>[2x]CGCAAATTXGCG

Using several techniques, we show that electron paramagnetic resonance (EPR) spectroscopy of oligonucleotides spin-labelled with triazole-appended nitroxides at the 2′ position offers a robust and minimally perturbing tool for obtaining such measurements. Here we address this challenge through a synergistic combination of EPR spectroscopy, X-ray crystallography, NMR spectroscopy and MD simulations, which accurately identify spin label location on a DNA duplex. As well as affording the first X-ray crystallographic structures of B-form spin-labelled DNA duplexes, the combination of these four techniques demonstrates the minimally perturbing nature of deoxynucleic acid 2′-spin-labelling. Using experimental and computational methods to support EPR spectroscopic observations, we demonstrate that spin-labelling of DNA via 2′-triazole-linked nitroxides is minimally perturbing and affords DEER data with narrow (sub-nanometre) distance distributions due to well-defined minor groove nitroxide conformations.

Copper-catalysed azide-alkyne cycloaddition with a tetramethylpyrrolinoxyl radical (‘5-Me’, 3) or a tetramethylpiperidinoxyl radical (‘6-Me’, 4) afforded duplexes 5 (containing two 5U modifications) and 6 (two 6U modifications). Notably, 6 adopts the B-form; prior to this work, the only reported crystal structure of spin-labelled DNA is in the A-form. The electron density of the 6-Me spin labels is well defined, with both modifications occupying the minor groove. The separation of the spin labels (measured from the centre of each N–O bond) is 2.87 nm, which is in good agreement with the most probable distance determined by EPR spectroscopy (2.99 nm). The electron density of all other residues is also well defined, except for the 5′-terminal 2′-deoxycytidines, whose base-pairing is disrupted by crystal-packing interactions with cobalt(III) hexammine ions and neighbouring duplexes in the crystal. Such crystal contacts are commonly observed in DNA structures containing both terminal CpG steps and cobalt ions and are thus not attributable to the inclusion of the spin labels, which are separated from the terminal residues by two intact base pairs. The triazole ring is oriented with a nitrogen atom positioned under the deoxyribose ring, which places the triazole carbon atoms and sidechain in a less hindered environment. Similarly, the piperidine C–C bonds at the linking carbon atom minimize steric interactions by adopting a gauche conformation relative to the N1–N2 bond of the triazole. In the second conformation, the labels orient antiparallel with respect to the helix, with the nitroxides solvent-exposed but close to the major groove (green, most probable distance 3.33 nm).>[2x]SMSTKSVLFGRPVQTEGVPNVYAGAPVVPWTPPEPGIDNLGINSIDTFAVPGVGEYTVAFDGWVRVVRSPSTSGEWADAEVYTNLIEMKMVGECEELGKITVTLNPDCLSAGQIRTPFDPYAGEGPSAKACRMAVGAIFDMPKLGLKLMNREPIILTIDDVRSIPPAGAPGKGQIYRMMPLLDVNDPDGQPVAYLTSLRFNMGGYLKPDQM

The high reactivity of enediynes with DNA makes them quite toxic. In natural environments, some microorganisms producing enediynes protect themselves from their cytotoxic action by a self-resistance mechanism that uses a self-sacrificing protein or specialized ABC transporters to export the toxin.

Access to the biosynthetic gene cluster of dynemicin has enabled the in vitro study of gene products within the cluster to decipher their roles in assembling this unique molecule. This paper reports the crystal structure of DynF, the gene product of one of the genes within the biosynthetic gene cluster of dynemicin. DynF is revealed to be a dimeric eight-stranded β-barrel structure with palmitic acid bound within a cavity. The structure of DynF was determined to a resolution of 1.50 Å with a final R work and R free of 0.16 and 0.19, respectively. The DynF crystal has two molecules in its asymmetric unit. An analysis of the crystal contacts with PISA predicts that DynF forms a stable dimer. DynF is comprised of antiparallel β-sheets that are connected by short loops and helical segments to form eight-stranded antiparallel β-barrels. The size and shape of the ligand, as well as its binding environment, are suggestive of a 16-carbon fatty acid, which was confirmed by gas chromatography–mass spectrometry (GC-MS) as palmitic acid.> MSPFPLTSMDKAFITVLEMTPVLGTEIINYRDGMGRVLAQDVYAKDNLPPFPASVKDGYAVRAADGPGDRFIIGESQAGEQPTQTVM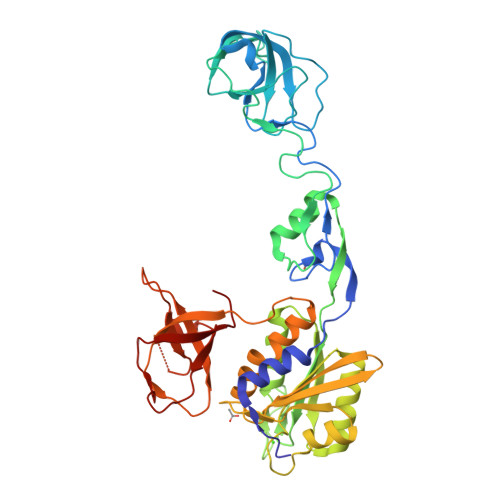PGQVMRVTTGAPIPCGADAVVQVEDTELIRESDDGTEELEVRILVQARPGQDIRPIGHDIKRGECVLAKGTHMGPSEIGLLATVGVTEVEVNKFPVVAVMSTGNELLNPEDDLLPGKIRDSNRSTLLATIQEHGYPTINLGIVGDNPDDLLNALNEGISRADVIITSGGVSMGEKDYLKQVLDIDLHAQIHFGRVFMKPGLPTTFATLDIDGVRKIIFALPGNPVSAVVTCNLFVVPALRKMQGILDPRPTIIKARLSCDVKLDPRPEYHRCILTWHHQEPLPWAQSTGNQMSSRLMSMRSANGLLMLPPKTEQYVELHKGEVVDVMVIGRL;>[2x]FSIVGSLPRDC> MSTSTYALRAGKRDVRREQQEIITRQINTAPYVQDAMMRVVVFAQYPSGRYKAFDYVFPDYLKVFLNWRELLEDTTTDYDPRTNTHRLMGQGYRQLIHPNHGSGEEPYDTRYPMGVIVSFNGNIDWTRARVEATNMHG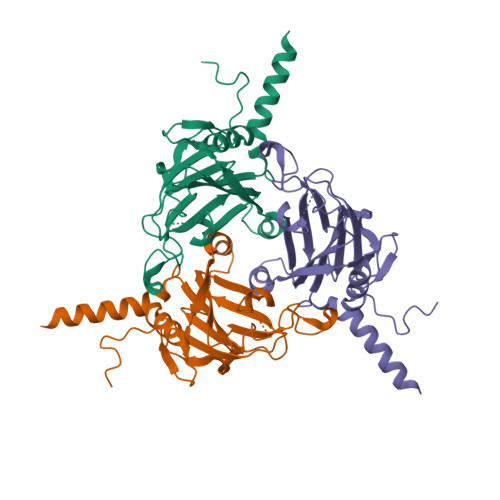LNNTDWREARAWGPHVICGNQLRKAGHLSRAVYVPLDEHNTVKVLATARQDGALNRFNGPQLAQTLTNNIVCPNVIEFNTESDVIDYAKMAHIAYIDQAGLIVASSDAYISGDSQA> ANLYFQSNAVVVYGADVICASCVNAPTSKDIYDWLQPLLKRKYPNISFKYTYIDITKDNDNLTDHDLQFIERIEQDELFYPLITMNDEYVADGYIQTKQITRFI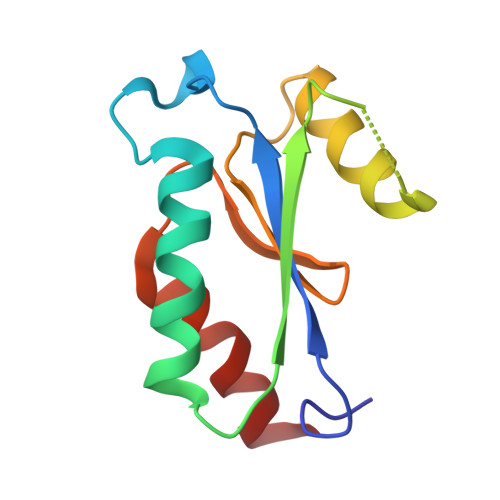DQKLVNE>[2x]MQLTPTFYDNSCPNVSNIVRDTIVNELRSDPRIAASILRLHFHDCFVNGCDASILLDNTTSFRTEKDAFGNANSARGFPVIDRMKAAVESACPRTVSCADLLTIAAQQSVTLAGGPSWRVPLGRRDSLQAFLDLANANLPAPFFT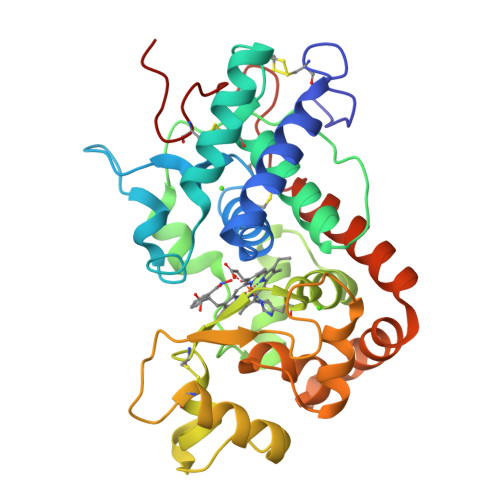LPQLKDSFRNVGLNRSSDLVALSGGHTFGKNQCRSIMDRLYNFSNTGLPDPTLNTTYLQTLRGLCPLNGNLSALVDFDLRTPTIFDNKYYVNLEEQKGLIQSDQELFSSPNATDTIPLVRSFANSTQTFFNAFVEAMDRMGNITPLTGTQGQIRLNCRVVNSNS> EFMEPKVAELKQKIEDTLCPFGFEVYPFQVAWYNELLPPAFHLPLPGPTLAFLVLSTPAMFDRALKPFLQSCHLRMLTDPVDQCVAYHLGRVRESLPELQIEIIADYEVHPNRRPKILAQTAAHVAGAAYYYQRQDVEADPWGNQRISGVCIHPRFGGWFAIRGVVLLPGIEVPDLPPRKPHDCVPTRADRIALLEGFNFHWRDWTYRDAVTP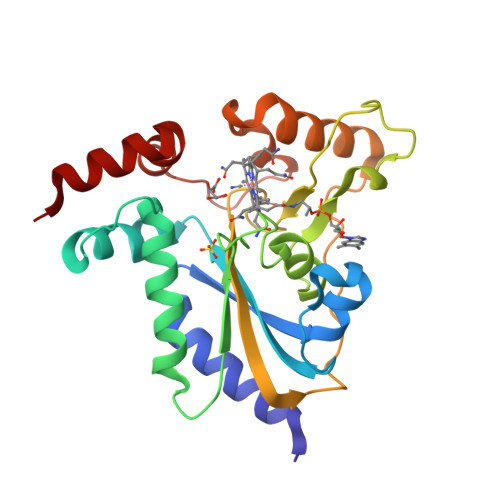QERYSEEQKAYFSTPPAQRLALLGLAQP>[6x]MTEAKIVDISSKDIVLREAVVEGYIKLRKETIEKIKNKEVEKGDVITVAKTAGILAAKKTPELIPMCHPIPLEFVDVEIKIEEEGLRVISTVKAHYKTGVEM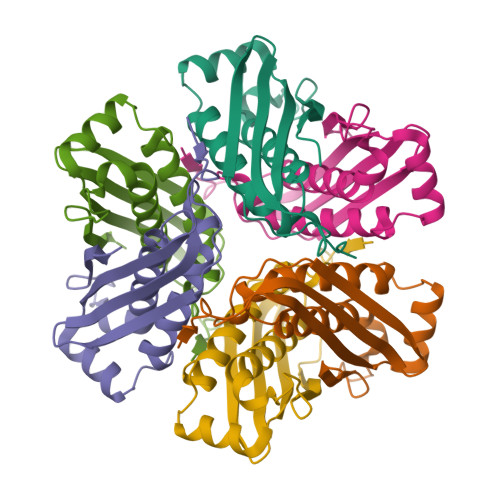EALTATSVALLTIWDMVKKYEKDENGQYPYTEIKSIRVINKIKTYDDMK>MHHHHHHELYLDTSDVVAVKALSRIFPLAGVTTNPSIIAAGKKPLDVVLPQLHEAMGGQGRLFAQVMATTAEGMVNDALKLRSIIADIVVKVPVTAEGLAAIKMLKAEGIPTLGTAVYGAAQGLLSALAGAEYVAPYVNRIDAQ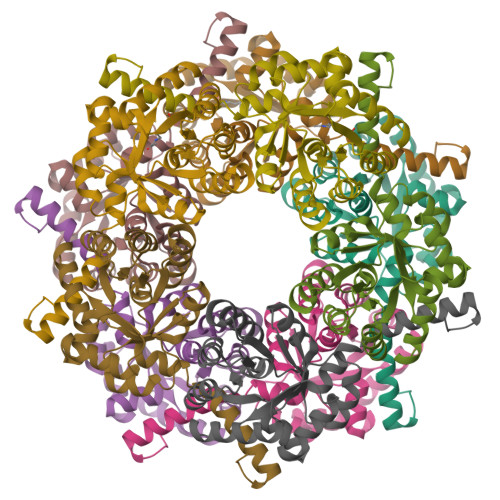GGSGIQTVTDLHQLLKMHAPQAKVLAASFKTPRQALDCLLAGCESITLPLDVAQQMISYPAVDAAVAKFEQDWQGAFGRTSI[20x]>MTVQDKAAGSDAEIVTALPVPLAVAGHHQPAPFYLTADMFGGLPVQLAGGELSKLVGKPVAAPHVHEVDELYFLVSPEPGQARIEVHLDGVRHELVSPAVMRIPAGSE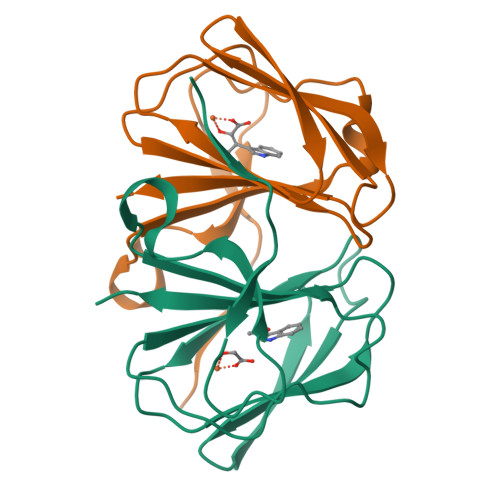HCFLTLEATVGSYCFGILVGDRL[2x]> MRRSLALCLHSTGACLLSAGKLSQYEQEAYESHRRFTESQTYPGPIRAATPGDTRFYMGSAETILQENERHYWRAVVDDPHVQHLVPLRVRFKTFIWVTSGWEQRVQVVQVMAQRDSTIAELMQQVRIENQSPYLCTSSFKLCIDGKDLDELKTLADYGIHEYSRIDAIEENDHLLHTEAERLKDWNVAEMPED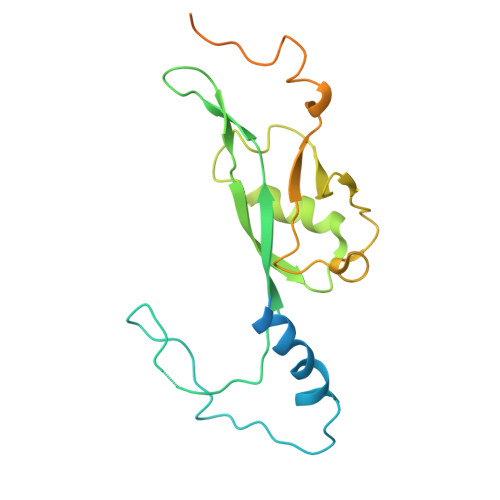VLLRSPYKEMAMQPQPNLAPRYEAKPKGYYGKNDYSGMKQSS>MIIWPSYIDKKKSRREGRKVPEELAIEKPSLKDIEKALKKLGLEPKIYRDKRYPRQHWEICGCVEVDYKGNKLQLLKEICKIIKGKN[2x];>MDKLGENLNKALNKLKAAAFVDKKLIKEVIKDIQRALIQADVNVKLVLKMSKEIERRALEEKTPKGLSKKEHIIKIVYEELVKLLGEEAKKLELNPKKQNVILLVGIQGSGKTTTAAKLARYIQKRGLKPALIAAD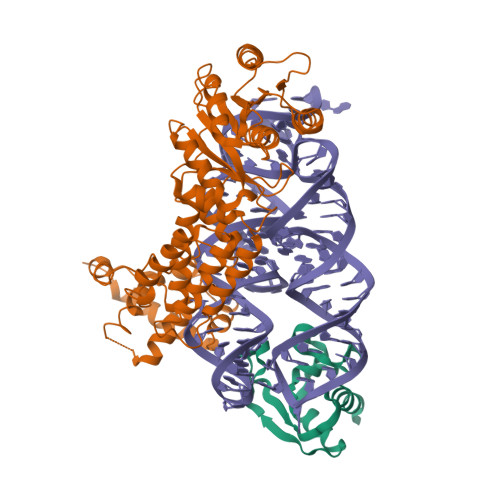TYRPAAYEQLKQLAEKIHVPIYGDETRTKSPVDIVKEGMEKFKKADVLIIDTAGRHKEEKGLLEEMKQIKEITNPDEIILVIDGTIGQQAGIQAKAFKEAVGEIGSIIVTKLDGSAKGGGALSAVAETKAPIKFIGIGEGIDDLEPFDPKKFISRLLGMGDLESLLEKAEDMVDEKTEESIDAIMRGKFTLNELMTQLEAIENMGSMKKILSMIPGFGGAMPKELSHLTEAKIKKYKVIISSMTKEERENPKIIKASRIRRIARGSGTTENDVREVLRYYETTKNAIDKLHHHHHH[2x]>[3x]GSHMDFVAFMNKINSINANLSRYENIINQIDAQHKDLLTQVSEEQEMELRRSLDDYISQATDLQYQLKADIKDAQRDGLHDSNKQAQAENCRQKFLKLIQDYRIIDSNYKEESKEQAKRQYTIIQPEATDEEVEAAINDVNGQQIFSQALLNANRRGEAKTALAEVQARHQELLKLEKTMAELTQLFNDMEELVIELTQLFNDMEELVIE;>QGHMSNFL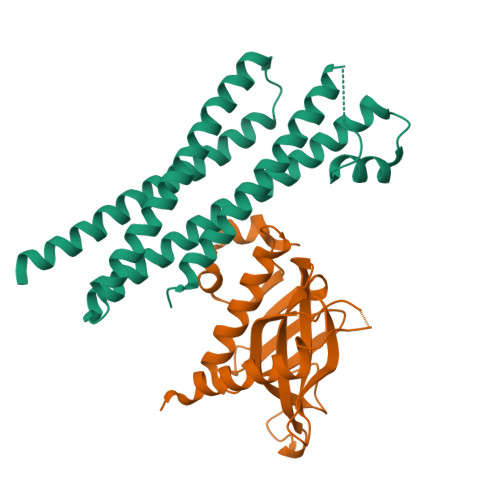AEQYERDRKAIINCCFSRPDHKTGEPPNNYITHVRIIEDSKFPSSRPPPDSKLENKKKRLLILSAKPNNAKLIQIHKARENSDGSFQIGRTWQLTELVRVEKDLEISEGFILTMSKKYYWETNSAKERTVFIKSLITLYIQTFEGHVPELVNWDLSLFYLDERSYQRAVITNRPGSVSPIKSPTSNFTTNTTQSVGSVPFSAPTERTRRSETESVNPVSTPASVEYHAGMKSLNKAPYSSNS[3x]>[3x]GTDERVYESIGQYGGETVKIVRIEKARDIPLGATVRNEMDSVIISRIVKGGAAE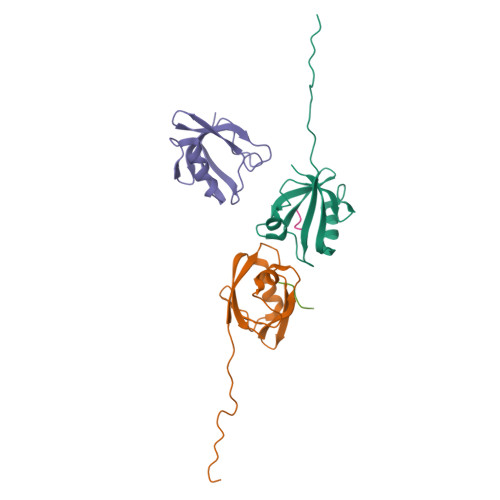KSGLLHEGDEVLEINGIEIRGKDVNEVFDLLSDMHGTLTFVLIPSQ;>NLNSSRVPDLLV[2x]>[4x]GSAMGSASTPQNPFQTPELKAFLERYNVTLHHQSGVNVDLGQDKEVDGKLYREAAGLCPVWGKYIQLHQPNRPPYKNNFLEDIPTEAEYQKSGNPLPGGFNMNFVTPAGQRISPYPMELLEKSSKIKASTELGKCAEFAYKTTAMDKSNQATQYRYPFVYDSKRRLC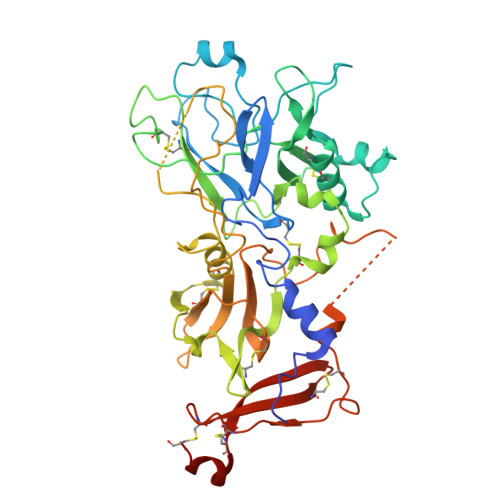YILSVSMQRMEGSKYCSTNDDPVNLTWYCFEPQKSPTANHNLIFGSAYVGKDPDAFLTKCPNQALKGYRFGHWTNGRCHDYTELADSWIEAVDSKAQCWVKTFTNDEVASDQPRTYPLTSQHSWNDWWPVHEKDQPHSGGDGRNYGFFYFDSNGKGKCALSHKAPDCLVSDSKAVSYTALGSLSEETPDIIIPSNPSVNPSTPDEALQCRSSEFPETFGSCDVQACKRQKTSCVGGQIQSTSVDCTAEEQNDCGSNTAAALVPR>[2x]MYPGSGNYSYNNRPSMPPPGFNGDGQGYRQEYGNQYGGGYQQQQYQDQYQGENRGQYQGQYQDQPEYGRPPSGMVRPPSSIQQGNGQQFQYSQMTGRRKALLIGINYIGSKNALRGCINDAHNIFNYLTTYCGYRPEDIVMLTDDQREMVKIPLKENIIRAMQWLVKDAQPNDALFFHYSGHGGQTKDLDGDEEDGMDDVIYPVDFESVGPLIDDTMHDIMVKSLPQGARLTALFDSCHSGTVLDLPYTYSTKGVIKEPNMWKDVGSDGIQAAMAYATGNRSALFSSIGNMVSSVTKKQNVDRERVRQIKFSPADVIMLSGSKDNQTSADTFADGQNIGAMSHAFISVMTRQPQQSYLSLLQNLRNELAGKYSQKPQLSASHPIDVNLQFIM

Metacaspases are caspase-like homologs which undergo a complex maturation process involving multiple intra-chain cleavages resulting in a composite enzyme made of a p10 and a p20 domain. Their proteolytic activity involving a cysteine-histidine catalytic dyad, show peptide bond cleavage specificity in the C-terminal to lysine and arginine, with both maturation- and catalytic processes being calcium-dependent. Here, we present the structure of a metacaspase from the yeast Candida glabrata, CgMCA-I, in complex with a unique calcium along with a structure in which three magnesium ions are bound. The monomers CgMCA-ICa and CgMCA-IMg both contain a p20 and a p10 domain forming a caspase-like core in which a two-stranded anti-parallel β-sheet from the p10 domain completes a six stranded parallel β-sheet in the p20 domain.

To determine the structure of CgMCA-ICa, we purified the wild-type metacaspase in the presence of 10 mM CaCl2 and performed crystallization assays at day 0 using a non-fully maturated protein. Crystals were observed only after three months, and the crystal structure reveals that the maturation process occurred in the course of the crystallization. Regarding the maturation process, the N-terminal and the linker located between p20 and p10 domains and which corresponds to the CgL6 loop, are both cleaved and residues Met1 to Gly68 and Asn260 to Ile309 show no electron density in the 2Fo-Fc map. Surprisingly, the two monomers of the CgMCA-ICa dimer observed in the asymmetric unit interact via a β-sheet complementation between the β6 and β5’ strands. This unexpected organization being similar to that of the dimer usually observed for caspases, SAXS experiments were performed to determine the oligomeric state of CgMCA-I in the presence of calcium and confirmed that this enzyme is monomeric in solution. In addition, as observed in the crystal structure of ScMCA-I16, loop CgL7 (named L3 in ScMCA-I), which may cap the substrate-binding groove, is disordered from Asp324 to Gly335. We observed a clear electron density for Ca2+. In CgMCA-ICa, Ca2+ is hepta-coordinated by a water molecule and residues Gly196, Asp198 (Asp173 in TbMCA-Ib), Asp214 (Asp189 in TbMCA-Ib), Thr242 and Asp245 (Asp220 in TbMCA-Ib). Interestingly, the “cation binding loop” observed in ScMCA-I (Gln223-Asp237) and in TbMCA-Ib (Cys162-Asp173) is ordered in CgMCA-ICa which suggests that the calcium has probably a role of stabilization not only for loop Asn185-Asp199 but also for segment Asp236- Asp245, the whole contributing to bringing together the two catalytic residues. Interestingly, in the presence of Mg2+ the distance between the two catalytic residues is 10.6 Å, against 8.3 Å when in presence of Ca2+, suggesting that the presence of calcium forces the catalytic site to adopt a proper organization for its autolysis activity.>[8x]TGGVQTVTLIPGDGIGPEISAAVMKIFDAAKAPIQWEERNVTAIQGPGGKWMIPSEAKESMDKNKMGLKGPLKTPIAAGHPSMNLLLRKTFDLYANVRPCVSIEGYKTPYTDVNIVTIRENTEGEYSGIEHVIVDGVVASIKLITEGASKRIAEFAFEYARNNHRSNVTAVHKANIMRMSDGLFLQKCREVAESCKDIKFNEMYLDTVCLNMVQDPSQFDVLVMPNLYGDILSDLCAGLIGGLGVTPSGNIGANGVAIFESVHGTAPDIAGKDMANPTALLLSAVMMLRHMGLFDHAARIEAACFATIKDGKSLTKDLGGNAKCSDFTEEICRRVKDLD;>ASRSQAEDVRVEGSFPVTMLPGDGVGPELMHAVKEVFKAAAVPVEFQEHHLSEVQNMASEEKLEQVLSSMKENKVAIIGKIHTPMEYKGELASYDMRLRRKLDLFANVVHVKSLPGYMTRHNNLDLVIIREQTEGEYSSLEHESARGVIECLKIVTRAKSQRIAKFAFDYATKKGRGKVTAVHKANIMKLGDGLFLQCCEEVAELYPKIKFETMIIDNCCMQLVQNPYQFDVLVMPNLYGNIIDNLAAGLVGGAGVVPGESYSAEYAVFETGARHPFAQAVGRNIANPTAMLLSASNMLRHLNLEYHSSMIADAVKKVIKVGKVRTSDMGGYATCHDFTEEICRRVKDLDEN[4x];>[4x]FSEQTIPPSAKYGGRHTVTMIPGDGIGPELMLHVKSVFRHACVPVDFEEVHVSSNADEEDIRNAIMAIRRNRVALKGNIETNHNLPPSHKSRNNILRTSLDLYANVIHCKSLPGVVTRHKDIDILIVR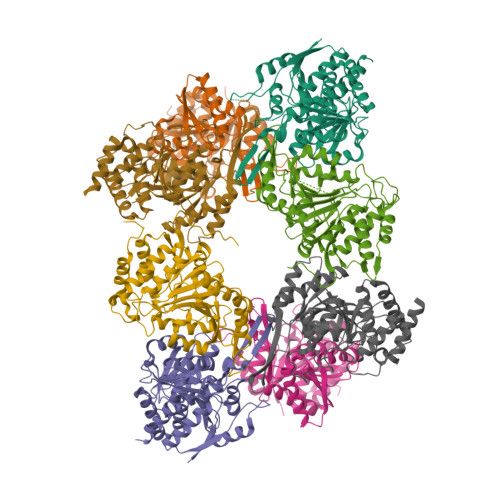ENTEGEYSSLEHESVAGVVESLKIITKAKSLRIAEYAFKLAQESGRKKVTAVHKANIMKLGDGLFLQCCREVAARYPQITFENMIVDNTTMQLVSRPQQFDVMVMPNLYGNIVNNVCAGLVGGPGLVAGANYGHVYAVFETATRNTGKSIANKNIANPTATLLASCMMLDHLKLHSYATSIRKAVLASMDNENMHTPDIGGQGTTSEAIQDVIRHIRVINGRAVEA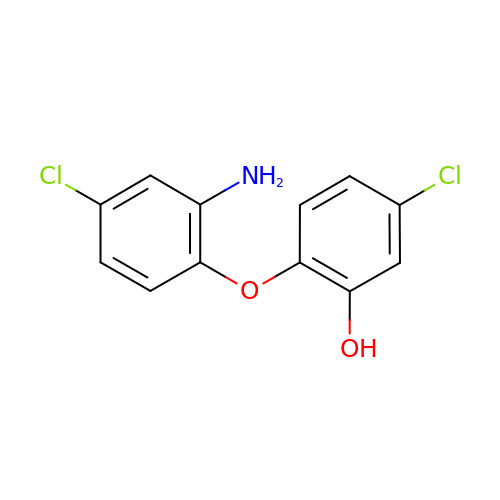2-(2-amino-4-chlorophenoxy)-5-chlorophenol | C12 H9 Cl2 N O2 | ZNHVVJUATLQYST-UHFFFAOYSA-N> MSTSLFSRTPKVTVFDNRGLTARDIAYHRHPDAPEVTNERITPHQYDARGFLTQSADPRLHDAGRVNFS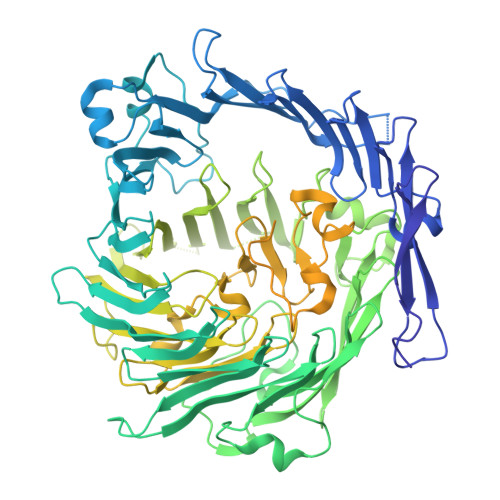YLTDLAGGVLRTQGADNGTSVSLNDVAGRPFIVVSHISATDEGTEDRSLAVTRTWQYEDAALPGRPLNVTEQISTEVARITERFVYAGNTGAEKTLNLAGLCVRHYDTAGLVQTDSIALTGVSLSVTRRLLKDADNPDTVADWQGEGASAWNDLLSGEEYVTLTTADATGTVLTTTDAKGNIQRVRYDVAGLLSGSWLTVRDRTEQVIVKSLTYSAAGQKQREDHGNGVVITYTYEAETQRLTGIRTERPAGHASGAKVLQDLRYEYDPVGNVLKITNDAEATRFWSNQKVVPENTYTYDSLYQLVSATGREMANVGQQGSRLPSATVPFPTDSSAYTSYTRTYTYDEASNLTQIRHSPATRSGYTTNITVSNRSNRAVLSNLTENAADVDALFTAGGQQTQLQPGLGLVWTARNELLKVTPVMRDGSADDSENYRYDGGSQRILKVSVQKTGNSAQTQRALYLPGLELRSAKNGDTETESLQVITVGEASRAQVRMLHWESGRPDGITDDKVRYSYDNLTGSSVLELDSDGKLISMEEYYPYGGTAVWTVRSAVEANYKTVRYSGKERDATGLYYYGYRYYQPWAGRWLSADPAGSVDGLNLYRMVRNNPVAWKDNDGRIPINTMIPPPPPMMGGNPPPPPPMMGGNPPPPPPVAGGNPPPPPSMPGQQNGAKKNWVIKEDPALYKQQGGEYPYYSSFTIALQKLNISHYDSIIDMDNFISKWAEIGRNMKPAARDISHDKFIEVQKTLGKIDAEWSGYHSADVNETFRGDTPVISNSYSWLAEFINESEGKSDTVQKSMDLEIKSPLIMSTAKDPKMGYVSGKTIMWHFDLEPGHAGVSEGLYASEGEVTFPLYNRMKITSLQYLPEGRSYMDNPEQYGTSHRYIIKARMLPRS4-O-methyl-alpha-D-glucopyranuronic acid | 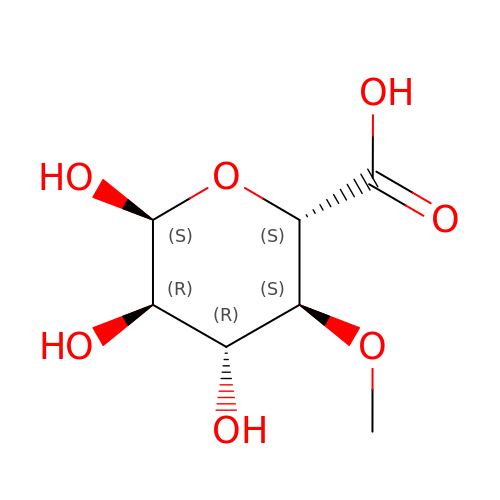C7 H12 O7 | WGLLPAPKWFDHHV-NRGGUMNKSA-N>[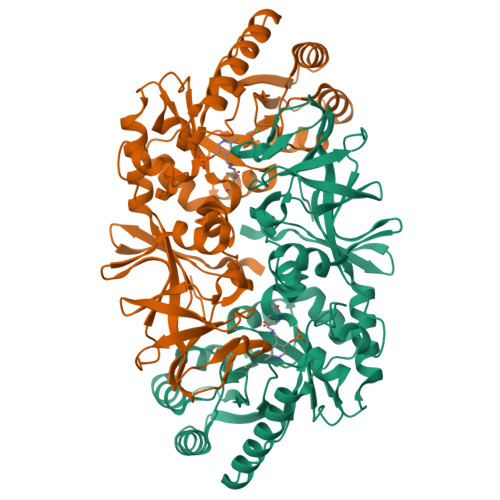2x]MEEAPFYRDTWVEVDLDAIYNNVTHIKEFIPSDVEIFAVVKGNAYGHDYVPVAKIALEAGATRLAVAFLDEALVLRRAGITAPILVLGPSPPRDINVAAENDVALTVFQKEWVDEAIKLWDGSSTMKYHINFDSGMGRIGIRERKELKGFLKSLEGAPFLELEGVYTHFATADEVETSYFDKQYNTFLEQLSWLKEFGVDPKFVHTANSAATLRFQGITFNAVRIGIAMYGLSPSVEIRPFLPFKLEPALSLHTKVAHIKQVIKGDGISYNVTYRTKTEEWIATVAIGYADGWLRRLQGFEVLVNGKRVPIVGRVTMDQFMIHLPCEVPLGTKVTLIGRQGDEYISATEVAEYSGTINYEIITTISFRVPRIFIRNGKVVEVINYLNDILEENLYFQ> MNFNVGVDFPSFIAWDGTTSFPVKIDGFNQFGFTFKVIEELTADVPFNIFYHEASEAD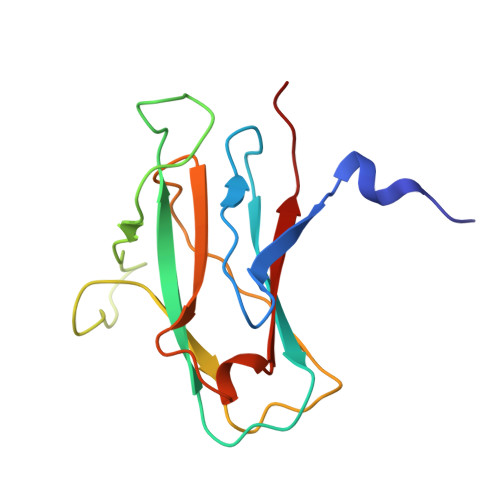PCVPGPAIRVPDVPFCDGVATADGLATVVIPEAVAVDSFCAGSVPCFNGPWISIAPVTVNADSAKVQVTVTMKGATR>[2x]GELETKAVGMSNDGRFLKFDIEIGRGSFKTVYKGLDTETTVEVAWCELQDRKLTKSERQRFKEEAEMLKGLQHPNIVRFYDSWESTVKGKKCIVLVTELMTSGTLKTYLKRFKVMKIKVLRSWCRQILKGLQFLHTRTPPIIHRDLKCDNIFITGPTG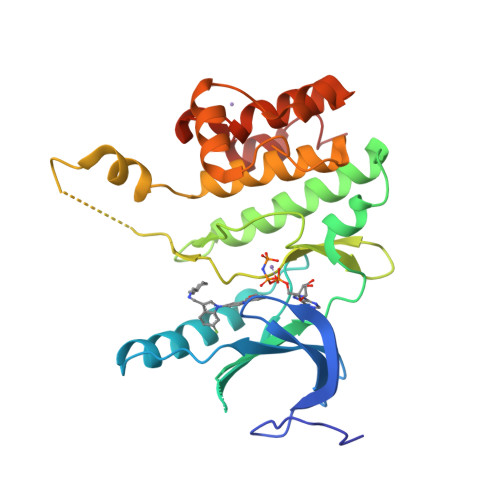SVKIGDLGLATLKRADFAKSVIGTPEFMAPEMYAAAYDESVDVYAFGMCMLEMATSEYPYSECQNAAQIYRRVTSGVKPASFDKVAIPEVKEIIEGCIRQNKDERYSIKDLLNHAFFQEET>MKKKGSVVIVGRINLSGDTAYAQQTRGEEGCQETSQTGRDKNQVEGEVQIVSTATQTFLATSINGVLWTVYHGAGTRTIASPKGPVTQMYTNVDKDLVGWQAPQGSRSLTPCTCGSSDLYLVTRHADVIPVRRRGDSRGSLLSPRPISYLKGSSGGPLLCPAGHAVGI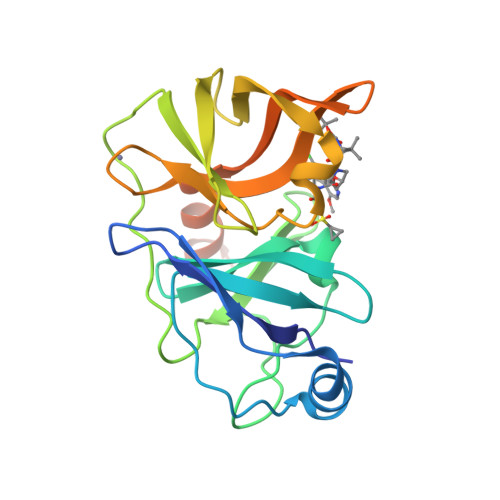FRAAVCTRGVAKAVDFIPVESLETTMRSPAIRAPSTSLRPHSSTTTTTTEI[2x]2-cyano-3-[5-(3-cyclohexyl-3,5,8,10-tetrazatricyclo[7.3.0.0^{2,6}]dodeca-1,4,6,8,11-pentaen-4-yl)furan-2-yl]-~{N},~{N}-dimethyl-prop-2-enamide | C24 H24 N6 O2 | 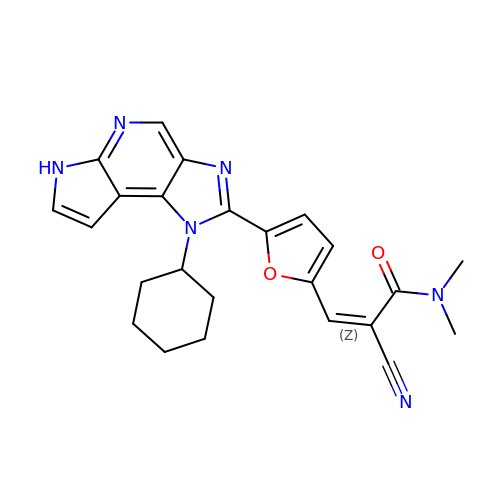GJMZWYLOARVASY-QINSGFPZSA-N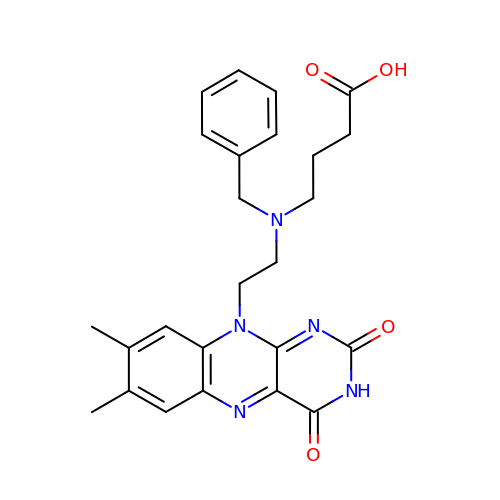4-{benzyl[2-(7,8-dimethyl-2,4-dioxo-3,4-dihydrobenzo[g]pteridin-10(2H)-yl)ethyl]amino}butanoic acid | C25 H27 N5 O4 | UHJZDXGBGFJXSS-UHFFFAOYSA-N> MSNITIYHNPACGTSRNTLEMIRNSGTEPTIILYLENPPSRDELVKLIADMGI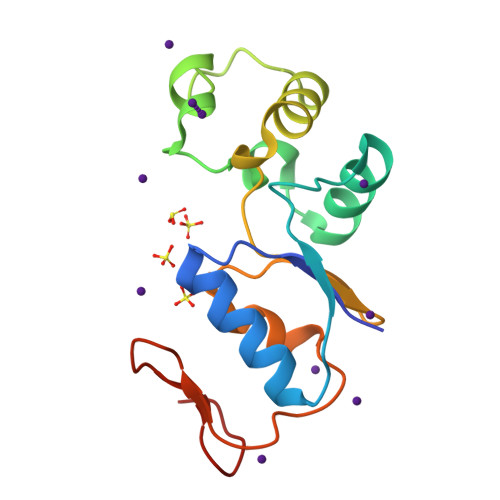SVRALLRKNVEPYEQLGLAEDKFTDDQLIDFMLQHPILINRPIVVTPLGTRLCRPSEVVLDILQDAQKGAFTKEDGEKVVDEAGKRLK COFORMYCIN 5'-PHOSPHATE | C11 H17 N4 O8 P 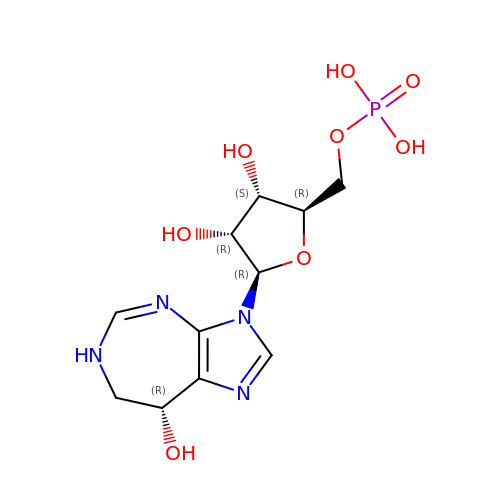| LWLMFZVGOXTQAI-LODYRLCVSA-N>GAMGSGIQMKEEASEHGGSADETQELSPVSDSSDEMPNNAKRRRRSQSMIANKRIHQAFQEDEGDEDWEEEEHKPKAKRRYNTRSNESFSEGDDEPFEVSESSALEDELSDSEDSFIRSVRSKPKYKPGTRRSTRLRNRRSQDEEESEEEHRPILRERTSRINYSVPLAFPPVDEMDGDPSSQVNQSRSRKTHSELAITKLLRQQVSSFMPYIDSSGSESESDNTRIKKSSAKTIKALTDPANSGGPPDFGRIREKSDLADSDPLGVDSSLSFESVGGLDNYINQLKEMVMLPLLYPEIFQRFNMQPPRGVLFHGPPGTGKTLMARALAAACSSENKKVSFYMRKGADCLSKWVGEAERQLRLLFEEAKSTQPSIIFFDQIDGLAPVRSSKQEQIHASIVSTLLALMDGMESRGQVIIIGATNRPDAVDPALRRPGRFDREFYFPLPDRDARKKIIEIHTRNWDPPVPEWLCSMLAEKSKGYGGADLRALCTEAALNSIKRTYPQLYRSTKRLQIDPKTIKVKVKDFVMSMKRMIPSSERSSISPSKPLSPELKPLLNEAFQDIEKTLQKLMPVASKLNPLEEVMYDDPKENDFEYQQRLETFETLRIYKPRFLICGRKGLGQTALGPAILQQYEGVHVQSFDMSTLLQDSTQSIETSIIHLFLEVRRHTPSIIYIPDIDNWLNVLPLTAITTFSSMLERLDFSDQILFLALSSSPLSELHPQLREWFSSKQSVYSLQYPTRDSIIAFFQPILELIKASPTELPGGIPRKRRVLPELPLAPDPPPFTSQKITLKQTKQADMRLLNKLKIKLNALLGSLRARYRKFKKPLIDFNDIYCVDPETGHSYRSREECHYEFVDDVVKQIGSDQKFSMMSLEEIEKRTWDNCYCTPKQFVHDIKLILRDALQLEDSETIKRAQEMYANVLLGVEDMEDDQFSQRCERMALREAERRKLRHGKLQKHLDETKADMQFTSEKPSVDESITEVDDAIKDGPPVLAETLTNSLMEDVGPENVDMDIEDNEIFTNQSTMSVPSM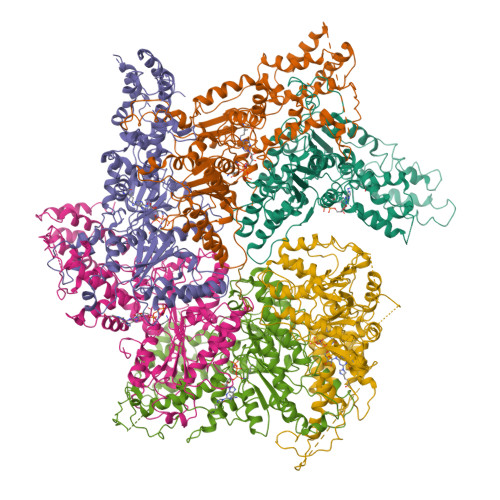LVENEESPKPDEYIDQKDKVQSPLLNGKSPVGVPSEAALRVSTDVSTNISSNGRADIPVDTLITSPADVPNNAPTDAHNITSADGHIENIEQEVVFPDLVFDEDRLTPLKQLLIDSTTGFTVDQLLHLHSFLYQIIWNTKSEWNRNSVVDECERAVKEFMINALQ[6x]>[2x]GSISTAVIDAINSGATLKDINAIPDDMMDDIYSYAYDFYNKGRIEEAEVFFRFLCIYDFYNVDYI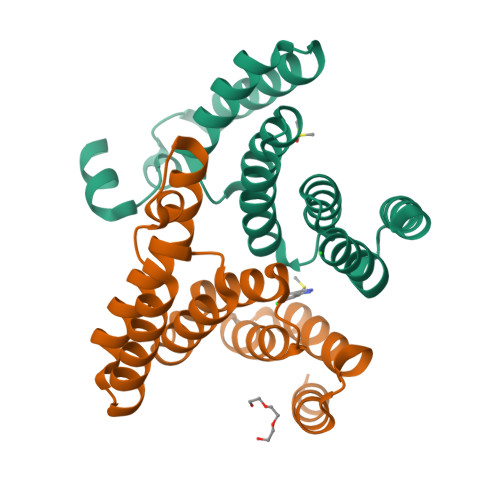MGLAAIYQIKEQFQQAADLYAVAFALGKNDYTPVFHTGQCQLRLKAPLKAKECFELVIQHSNDEKLKIKAQSYLDAIQ Adaptor protein complex 2 α and β-appendage domains act as hubs for the assembly of accessory protein networks involved in clathrin-coated vesicle formation. The C-terminal “appendage domains” of the large subunits recruit interaction partners from the cytosol facilitating their concentration at sites of coated pit formation. We identify a large repertoire of β-appendage interactors by mass spectrometry. These interact with two distinct ligand interaction sites on the β-appendage (the “top” and “side” sites) that bind motifs distinct from those previously identified on the α-appendage. We solved the structure of the β-appendage with a peptide from the accessory protein Eps15 bound to the side site and with a peptide from the accessory cargo adaptor β-arrestin bound to the top site.

We obtained co-crystals for Eps15 P-short peptide (SFGDGFADFSTL) with the β-appendage and see density for the complete peptide. The peptide forms a tight turn with the side-chains of F2 and F9 in a groove and that of F6 lying against a shallow pocket. The tight turn is formed by G5, and the psi and phi angles for this residue lie in a region of the Ramachandran plot permitted only for glycine residues. The turn is stabilised by the side chain of D8: it forms hydrogen bonds with the backbone nitrogen atoms of G3 and G5. The D8 side chain also forms a hydrogen-bond with Y815 of the appendage giving specificity to the peptide. F2 is surrounded by N758, Q804, V805, A806 and Y815 where A806 is found in the base of the groove. F9 projects into a shallow pocket lined by A754, Q756, K808, and V813. There were two β-appendage molecules in the asymmetric unit and consequently the peptide binding sites are in different crystallographic environments. The peptide we describe (that bound to molecule A) is sandwiched between the two molecules but is mostly bound to A. There are a few stabilising interactions with residues from B. We observe hydrogen bonds from the backbone nitrogen of chain B L819 and the ring nitrogen of chain B W714 to the side chain of D4 along with some other interactions via water molecules, as well as some interactions with the partially exposed F6. Mutagenesis of this site confirms that Y815 on the β-appendage is a critical residue presumably as it π stacks with F2 and H-bonds to D8.

>IGMAPGGYVAPKAVWLPAVKAKGLEISGTFTHRQGHIYMEMNFTNKALQHMTDFAIQFNKNSFGVIPSTPLAIHTPLMPNQSIDVSLPLNTLGPVMKMEPLNNLQVAVKNNIDVFYFSCLIPLNVLFVEDGKMERQVFLATWKDIPNENELQFQIKECHLNADTVSSKLQNNNVYTIAKRNVEGQDMLYQSLKLTNGIWILAELRIQPGNPNYTLSLKCRAPEVSQYIYQVYDSILKN[2x];> SFGDGFADFSTL>[12x]MCRHVAWLGAPRSLADLVLDPPQGLLVQSYAPRRQKHGLMNADGWGAGFFDDDGVARRWRSDKPLWGDASFASVAPALRSRCVV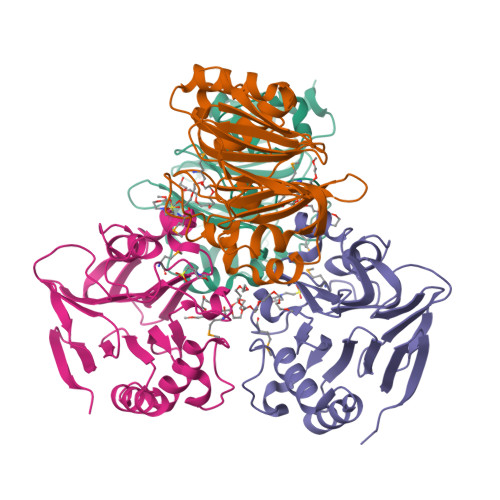AAVRSATIGMSIEPSASAPFSDGQWLLSHNGLVARGVLPLTGAAESTVDSAILAALIFSRGLDALGATIAEVGELDPNARLNILAANGSRLLATTWGDTLSVLRRPDGVVLASEPYDDDPGWSDIPDRHLVDVRDAHVVVTPLSSHHHHHH>[2x]KPKLHYFNARGRMESTRWLLAAAGVEFEEKFIKSAEDLDKLRNDGYLMFQQVPMVEIDGMKLVQTR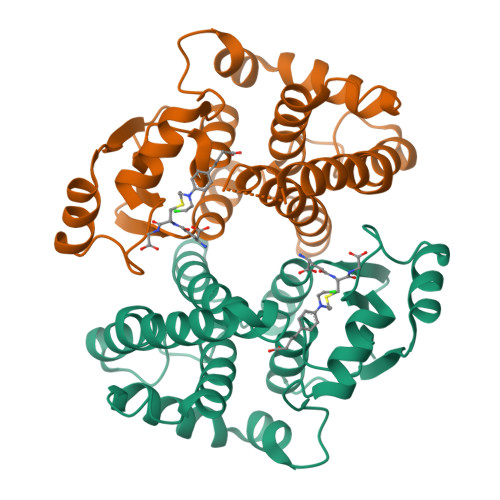AILNYIASKYNLYGKDIKERALIDMYIEGIADLGEMILLLPVCPPEEKDAKLALIKEKIKNRYFPAFEKVLKSHGQDYLVGNKLSRADIHLVELLYYVEELDSSLISSFPLLKALKTRISNLPTVKKFLQPGSPRKPPMDEKSLEEARKIF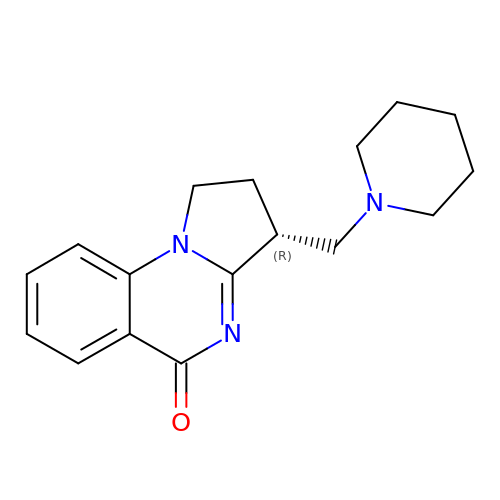(3~{R})-3-(piperidin-1-ylmethyl)-2,3-dihydro-1~{H}-pyrrolo[1,2-a]quinazolin-5-one | C17 H21 N3 O | CDOMBRFDONICCK-CYBMUJFWSA-N> GEKKECWSWESYLEEQKAITAPVSLFQDSQAVTHNKNGFKLGMKLEGIDPQHPSMYFILTVAEVCGYRLRLHFDGYSECHDFWVNANSPDIHPAGWFEKTGHKLQPPKGYKEEEFSWSQYLRSTRAQAAPKHLFVSQSHSPPPLGFQVGMKLEAVDRMNPSLVCVASVTDVVDSRFLVHFDNWDDTYDYWCDPSSPYIHPVGWCQKQGKPLTPPQDYPDPDNFCWEKYLEETGASAVPTWAFKVRPPHSFLVNMKLEAVDRRNPALIRVASVEDVEDHRIKIHFDGWSHGYDFWIDADHPD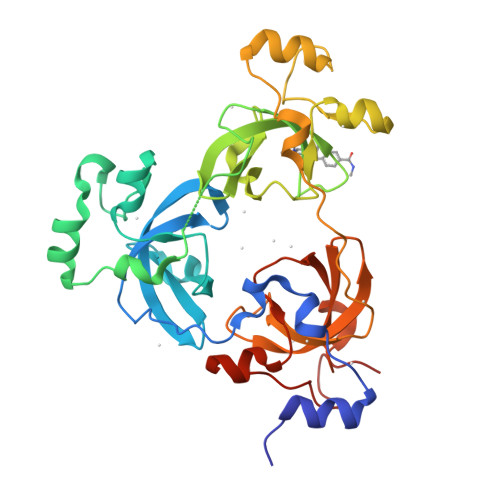IHPAGWCSKTGHPLQPPLGPREPSSASPGG>[2x]MGSSHHHHHHSSGLVPRGSTSEVIEDEKQFYSKAKTYWKQIPPTVDGMLGGYGHISSIDINSSRKFLQRFLREGPNKTGTSCALDCGAGIGRITKRLLLPLFREVDMVDIT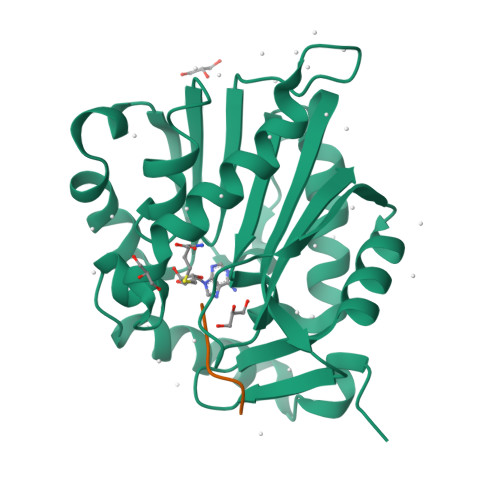EDFLVQAKTYLGEEGKRVRNYFCCGLQDFTPEPDSYDVIWIQWVIGHLTDQHLAEFLRRCKGSLRPNGIIVIKDNMAQEGVILDDVDSSVCRDLDVVRRIICSAGLSLLAEERQENLPDEIYHVYSFALR;>[2x]YPKRIA Isovaleryl-coenzyme A | C26 H44 N7 O17 P3 S | 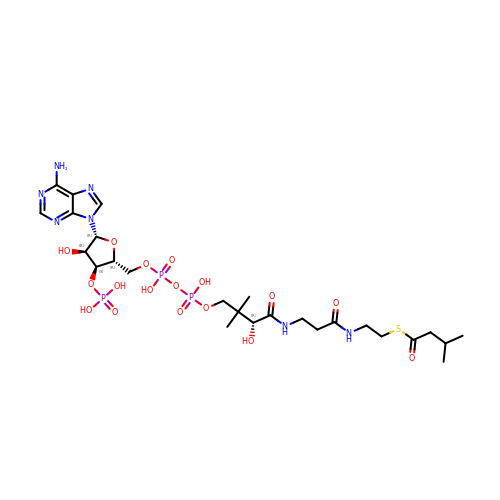UYVZIWWBJMYRCD-ZMHDXICWSA-N>[2x]MKSKFKLTTAAAMLGLMVLAGGAQAQDKPREVLTGGHSVS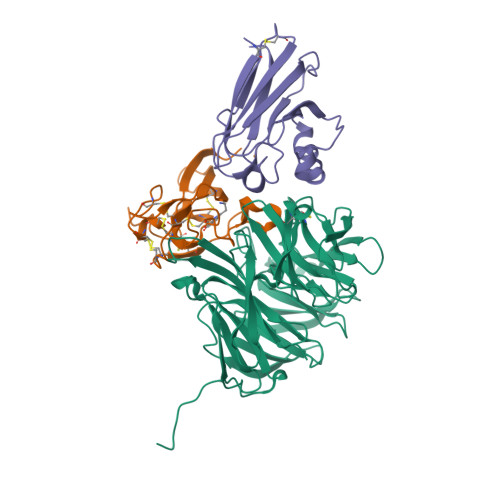APQENRIYVMDSVFMHLTESRVHVYDYTNGKFLGMVPTAFNGHVQVSNDGKKIYTMTTYHERITRGKRSDVVEVWDADKLTFEKEISLPPKRVQGLNYDGLFRQTTDGKFIVLQNASPATSIGIVDVAKGDYVEDVTAAAGCWSVIPQPNRPRSFMTICGDGGLLTINLGEDGKVASQSRSKQMFSVKDDPIFIAPALDKDKAHFVSYYGNVYSADFSGDEVKVDGPWSLLNDEDKAKNWVPGGYNLVGLHRASGRMYVFMHPDGKEGTHKFPAAEIWVMDTKTKQRVARIPGRDALSMTIDQQRNLMLTLDGGNVNVYDISQPEPKLLRTIEGAAEASLQVQFHPVGGV;>AGGGGSSSGADHISLNPDLANEDEVNSCDYWRHCAVDGFLCSCCGGTTTTCPPGSTPSPISWIGTCHNPHDGKDYLISYHDCCGKTACGRCQCNTQTRERPGYEFFLHNDVNWCMANENSTFHCTTSVLVGLAKN[2x];> ACDVSIEGNDSMQFNTKSIVVDKTCKEFTINLKHTGKLPKAAMGHNVVVSKKSDESAVATDGMKAGLNNDYVKAGDERVIAHTSVIGGGETDSVTFDVSKLKEGEDYAFFCSFPGHWSIMKGTIELGS>[3x]ATMITSNQLGTITEDSGSYTPGTIATATRLVLTPRETPQSITVVTRQNMDDFGLNNIDDVMRHTPGITVSAYDTDRNNYYARGFSINNFQYDGIPSTARNVGYSAGNTLSDMAIYDRVEVLKGATGLLTGAGSLGATINLIRKKPTHEFKGHVELGAGSWDNYRSELDVSGPLTESGNVRGRAVAAYQDKHSFMDHYERKTSVYYGILEFDLNPDTMLTVGADYQDNDPKGSGWSGSFPLFDSQGNRNDVSRSFNNGAKWSSWEQYTRTVFANLEHNFANGWVGKVQLDHKINGYHAPLGAIMGDWPAPDNSAKIVAQKYTGETKSNSLDIYLTGPFQFLGREHELVVGTSASFSHWEGKSYWNLRNYDNTTDDFINWDGDIGKPDWGTPSQYIDDKTRQLGSYMTARFNVTDDLNLFLGGRVVDYRVTGLNPTIRESGRFIPYVGAVYDLNDTYSVYASYTDIFMPQDSWYRDSSNKLLEPDEGQNYEIGIKG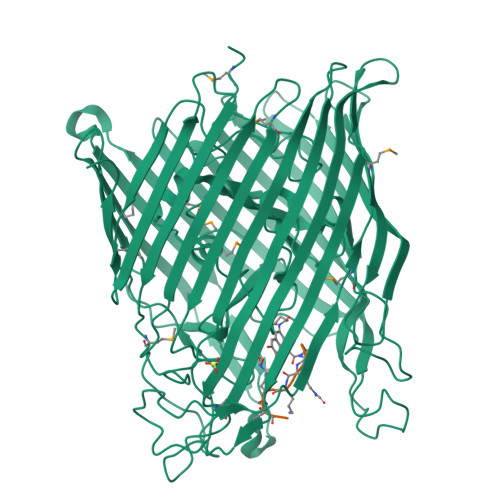EYLDGRLNTSLAYFEIHEENRAEEDALYNSKPTNPAITYAYKGIKAKTKGYEAEISGELAPGWQVQAGYTHKIIRDDSGKKVSTWEPQDQLSLYTSYKFKGALDKLTVGGGARWQGKSWQMVYNNPRSRWEKFSQEDYWLVDLMARYQITDKLSASVNVNNVFDKTYYTNIGFYTSASYGDPRNLMFSTRWDF;>SRSKKKTT[3x]> MITMKCRKCGKPSIYHQKHSGNNYCKECFIKETKRKVRKTLGRDVLKNNIKVAMGLSGGKDSLVMAYLL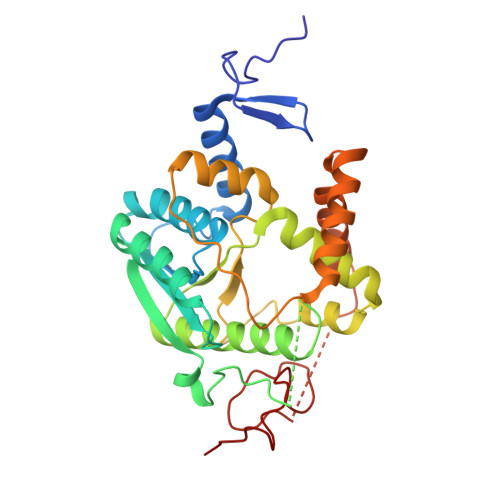NEYYKQIPNSNLIAIMVNEGIEGYRTDGIDAAVKFCEEYGIEYKIVHFKDYLGTNLDEIVKIAKEKNLTMNPCSFCGVIRRKILNRVSIEEKCDFLAIGHNLDDVAQAVMMNYIEGDVKKLAFLGKSLKHPKFVKRIKPLEKIPEDEVLLLAEMLELKYHKSPCPYSCLSFRSEVSDITDNLEKNHPGSKYSIVRGYERLLEHIELPGYTGECKICGDLSATEVCKVCSYLKNLGILEK> MRQVW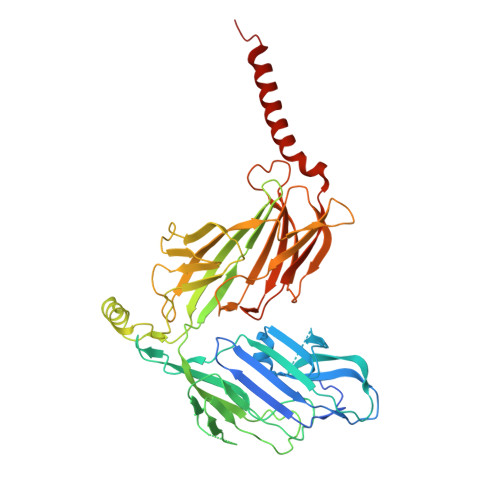FSWIVGLFLCFFNVSSAAQYEPPATWENVDYKRTIDVSNAYISETIEITIKNIASEPATEYFTAFESGIFSKVSFFSAYFTNEATFLNSQLLANSTTAPGDDGESEIRYGIIQFPNAISPQEEVSLVIKSFYNTVGIPYPEHVGMSEEQHLLWETNRLPLSAYDTKKASFTLIGSSSFEEYHPPNDESLLGKANGNSFEFGPWEDIPRFSSNETLAIVYSHNAPLNQVVNLRRDIWLSHWASTIQFEEYYELTNKAAKLSKGFSRLELMKQIQTQNMRQTHFVTVLDMLLPEGATDHYFTDLVGLVSTSHAERDHFFIRPRFPIFGGWNYNFTVGWTNKLSDFLHVSSGSDEKFVASIPILNGPPDTVYDNVELSVFLPEGAEIFDIDSPVPFTNVSIETQKSYFDLNKGHVKLTFSYRNLISQVANGQVLIKYDYPKSSFFKKPLSIACYIFTALMGVFVLKTLNMNVTN>GHMVPELKQISREEAMRLGPGWSHSCHAMLYAANPGQLFGRIPMRFSVLMQMRFDGLLGFPGGFVDRRFWSLEDGLNRVLGLGLGGLRLTEADYLSSHLTEGPHRVVAHLYARQLTLEQLHAVEISAVHSRDHGLEVLGLVRVPLYTQKDRVGGFPNFLSNAFVSTAKYQLLFALKVLNMMPSEKLAEALASATEKQKKALEKLLPPSS[2x];> GHMNSFVGLRVVAKWSSNGYFYSGKITRDVGAGKYKLLFDDGYECDVLGKDILLCDPIPLDTEVTALSEDEYFSAGVVKGHRKESGELYYSIEKEGQRKWYKRMAVILSLEQGNRLREQYGLG

The tumor suppressor p53-binding protein 1 (53BP1) plays a pivotal role in orchestrating the choice of DSB repair pathway. Central to the 53BP1 function is the recruitment of 53BP1 to the damaged chromatin via the recognition of di-methylated lysine 20 of histone H4 (H4K20me2) and ubiquitinated lysine 15 of histone H2A (H2AK15ub). More recently, a Tudor-interacting repair regulator (TIRR) has been characterized as a novel 53BP1 regulator, which directly binds to 53BP1 Tudor domain and blocks its H4K20me2 binding surface. In this study, we report the high-resolution structure of TIRR in complex with the tandem Tudor domain of 53BP1.

The crystal structure of the complex reconstituted with mouse TIRR and 53BP1 Tudor at 2:1 molar ratio is determined at 1.76-Å resolution by molecular replacement. In the complex structure, a TIRR monomer comprises seven α-helices (α1–α7) and seven β-strands (β1–β7), whereas 53BP1 Tudor comprises two α-helices (α1–α2) and ten β-strands (β1–β5, β1′–β5′). It is worth noting that the binding of one 53BP1 Tudor to TIRR dimer does not block the Tudor-binding site on the unbound TIRR protomer, suggesting that two molecules of 53BP1 could in theory bind to one TIRR dimer. The complex structure shows that the N-terminal region (residues 10–24) and the L8-loop of TIRR are engaged with a concave surface of 53BP1 Tudor, which is delineated by three loops (L1, L3, and L1′) of 53BP1 Tudor. While the N-terminal region of TIRR engaged with the L1-loop and L3-loop of 53BP1 Tudor, TIRR L8-loop mainly interacted with the 53BP1 Tudor L1′-loop. TIRR residues I12, L20, and W24 in the N-terminal region, together with residue L101 in β5-strand, engage with 53BP1 residues W1495, Y1523. In brief, TIRR residues P105, H106 form hydrophobic cluster with 53BP1 residues Y1500, Y1502 in L1 loop and L1547, and F1553 in L1′ loop. We observed that H4K20me2-bound aromatic cage, which contains 53BP1 residues W1495, Y1523, D1521, Y1502, and F1519, undergoes conformational changes upon TIRR interaction. In particular, residues W1495 and Y1523 display the largest conformational change and completely alter the structure of the aromatic cage. TIRR uses its N-terminal region coupled with L8-loop to block the methylation reader binding surface in Tudor, thus abolishing the access of 53BP1 to nucleosome bearing H4K20me2.>AYVCREASISGEIRYPQGTCPTKTEALNDCNKVTKGLIDFSQSHQRAWGIDMTAKVQCAPCKTTDPWDVVLCTCKITAHRYREFVPKIPYSSFSSAPGVIFRQETGLDHDPEWVVNMKARTRGCDHHH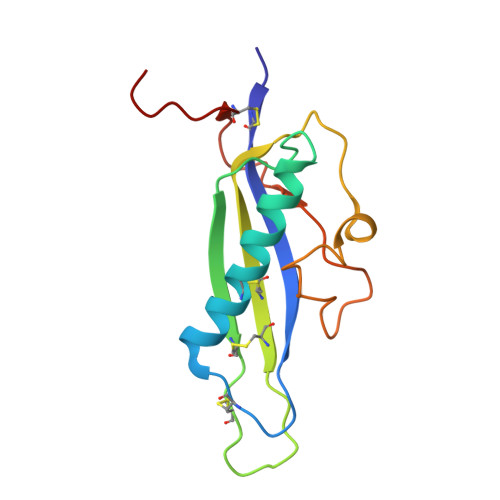HHH[4x]5-hydroxy-2-methylnaphthalene-1,4-dione | C11 H8 O3 | 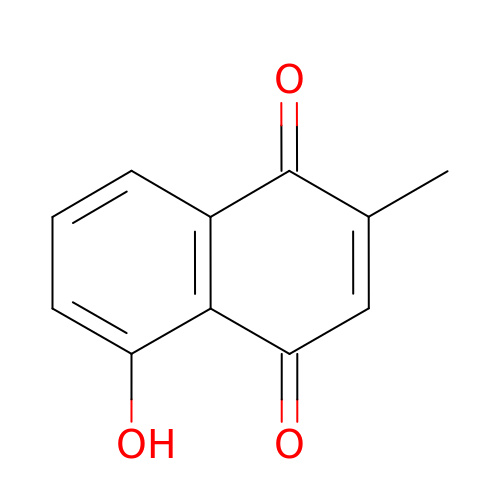VCMMXZQDRFWYSE-UHFFFAOYSA-N>GGUGGUGAAGUCGCUGG[2x];>[2x]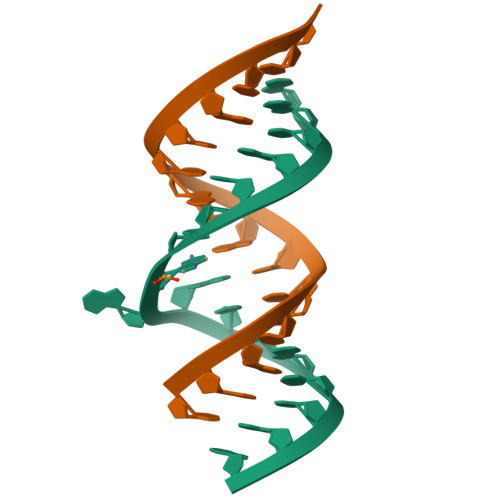CAGCGUCACACCACCC>MDDLTIEILTDDADYDLQRFDCGEEALNLFLTTHLVRQHRNKILRAYILCRNTPERQVLGYYTLCGSCFERAALPSKSKQKKIPYKNIPSVTLGRLAIDRSLQGQGWGATLVAHAMNVVWSASLAVGIHGLFVEALNEKAHTFYKSLGFIPLVGENENALFFPTKSIELLFT[2x];>[4x]KQRIDLRLTDDDKSMI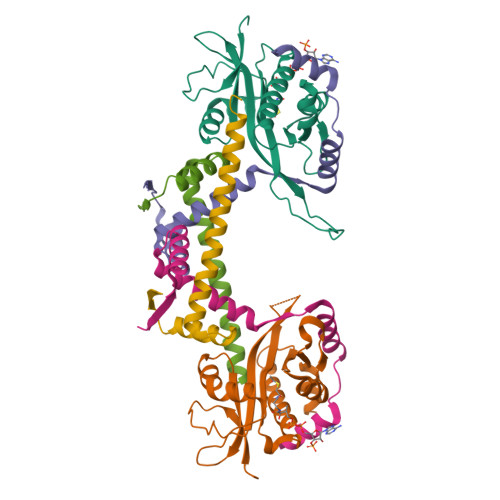EEAAAISNQSVSQFMLNSASQRAAEVIEQHRRVILNEESWTRVMDALSNPPSPGEKLKRAAKRLQ> ANPLYQKHIISINDLSRDDLNLVLATAAKLKANPQPELLKHKVIASCFFEASTRTRLSFETSMHRLGASVVGFSDSANTSLGKKGETLADTISVISTYVDAIVMRHPQEGAARLATEFSGNVPVLNAGDGSNQHPTQTLLDLFTIQETQGRLDNLHVAMVGDLKYPRTVHSLTQALAKFDGNRFYFIAPDALAMPQ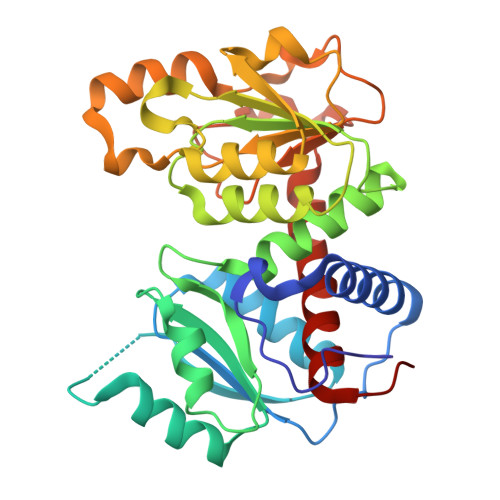YILDMLDEKGIAWSLHSSIEEVMAEVDILYMTRVQKERLDPSEYANVKAQFVLRASDLHNAKANMKVLHPLPRVDEIATDVDKTPHAWYFQQAGNGIFARQALLALVLNRDLVL> GAQVSTQKTGAHETSLSAAGNSIIHYTNINYYKDAASNSANRQDFTQDPSKF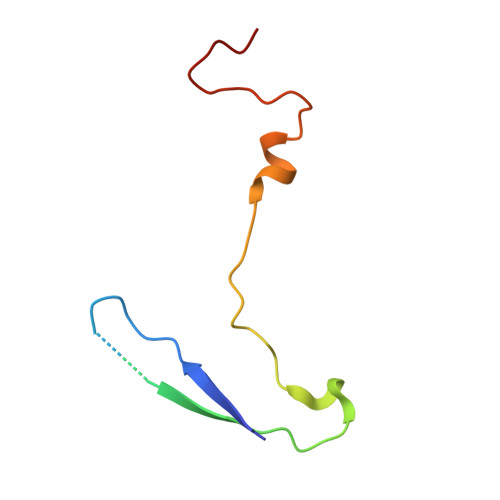TEPVKDVMIKSLPALN Here, we determined an X-ray crystal structure and performed functional analyses of two rice 2ODD family enzymes, OsGA2ox3 and OsDAO, which catabolize plant growth hormones GA4 and IAA, respectively. Both enzymes formed tetramers for OsGA2ox3, and dimers for OsDAO with the aid of their substrates, thereby enhancing their activity, as schematically summarized in Fig. 5c. With increasing substrate concentration, the enzyme gradually forms a multimer with the aid of the substrate itself (effecter), thereby resulting in an increase in enzymatic activity and in the active catabolism of GA or IAA to maintain hormonal homeostasis. The results revealed that a monomer–multimer switching occurs based on a substrate level, and that the resulting conformational change enhances the activities of these enzymes to maintain phytohormone homeostasis, in full agreement with the allosteric theory by Monod and co-workers.

We elucidated the crystal structure of OsDAO complexed with its substrate, IAA, at a 2.0-Å resolution. As expected, OsDAO had a stereotype structure of 2ODD, and formed a dimer containing two IAA molecules at the interface region. An IAA contacting subunit A (green stick) interacted with R154 and S176 of subunit A and R282 of subunit B via a water molecule, while the other IAA on subunit B (cyan stick) interacted with R281, R290, and S176 of subunit B and R282 of subunit A. These subunits directly interacted with each other through hydrogen bonds at residues D278, D279, R281, and R282. The elution profile of gel filtration showed that dimer formation of OsDAO occurred in the presence of IAA but not in its absence. Km for IAA of the dimer was nearly fivefold lower than that of the monomer, while consistently, Vmax of the dimer was 22-fold higher than that of the monomer. These observations demonstrated that the activity of an auxin-catabolizing enzyme, DAO, is regulated by the same mechanism that regulates GA2ox; namely, through substrate-mediated multimerization. Recent studies have revealed that DAO controls IAA concentration, which is important for modulating auxin homeostasis, since it is dependent on catabolizing IAA. Interestingly, all DAOs listed in Supplementary Fig. 10 share Arg or Lys at residue 308 in OsGA2ox3, which is essential for GA4-dependent oligomerization and hyperactivation, as previously mentioned.

>[2x]MVEIPAIDLRLAGGGGGAEETARLRDACARLGCFRVSGHGVPPGLQAEMKAAVRALFDLPDDAKRRNADIIPGSGYVPPGTANPLYEAFGLCDAAAPADVDAFCARLDAPPHVRETVKAYAERMHSLIVDVAGKVAASLGLHGASFQDWPCQFRMNRYNYTQDSVGSPGVQVHTDSGFLTVLQEDECVGGLEVLDPAAGEFVPVDPLPGSFVVNVGDVGQAWSNGRLHNVKHRVQCVAAVPRVSIAMFLLAPKDDTVSAPGELVDGEHPRRYREFKYDDYRRLRLSTGERAGEALARLAA> HMPVFEDVTRALVRELNPRGDLTPLDSLIDFKHFRPFCLVLRKRKSTLFWGARYVRTDYTLLDLLEPGSSPSDLTDSGNFSFKNMLDVQVQGLVEVPKTVKVKGTAGLSQSSTLEVQTLSVAPSALENLKKERKLSADHSFLNEMRYHEKNLYVVMEAVEAKQEVTVEQTGNANAIFSLPSLALLGLQGSLNNNKAVTIPKGCVLAYRVRLLRVFLFNLWDIPYICNDSMQTFPKIRRVPCSAFISP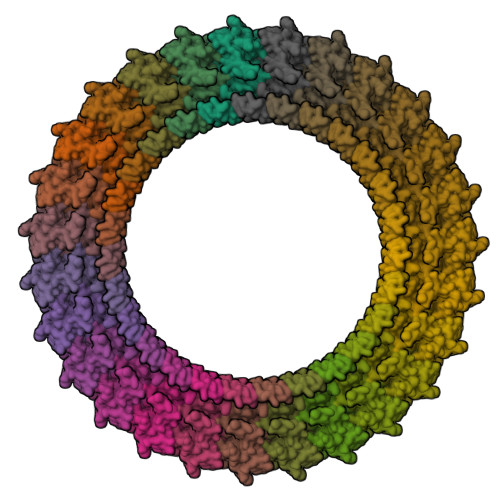TQMISEEPEEEKLIGELEVLFQ>[3x]AKCVSYGVSQIKAPALHSQGYTGSNVKVAVIDSGIDSSHPDLNVAGGASFVPSETNPFQDNNSHGTHVAGTVLAVAPSASLYAVKVLGADGSGQYSWIINGIEWAIANNMDVINMSLGGPSGSAALKAAVDKAVASGVVVVAAAGNSGTSGSSSTVSYPAKYPSVIAVGAVDSSNQRAPWSSVGPELDVMAPGVSICSTLPGNKYGAHDGTCPASNHVAGAAALIL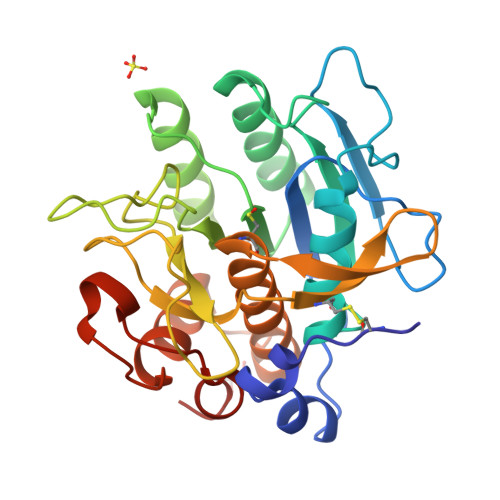SKHPNWTNTQVRSSLENTATKLGDSFYYGKGLINVEAAAQHHHHHH;> LPEGSPVTLDLRY> GPGSMSCYNEITTLLE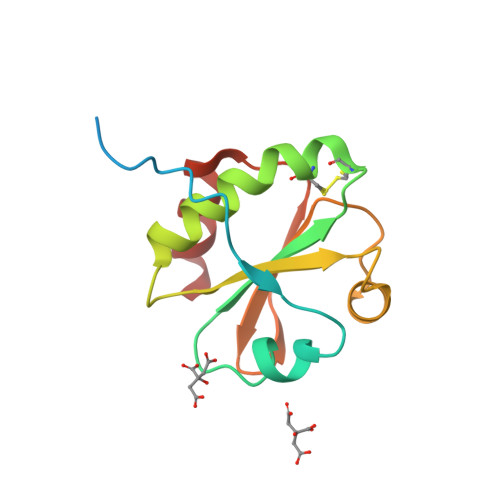FDSNDINTTQRINMVNNVTDSSFKNEVLESDLPVMVDFWAEWCGPCKMLIPIIDEISKELQDKVKVLKMNIDENPKTPSEYGIRSIPTIMLFKNGEQKDTKIGLQQKNSLLDWINKSI> GPHMLNPQLVQPAKKPYNKIVSHLLVAEPEKIYAMPDPTVPDSDIKALTTLCDLADRELVVIIGWAKHIPGFSTLSLADQMS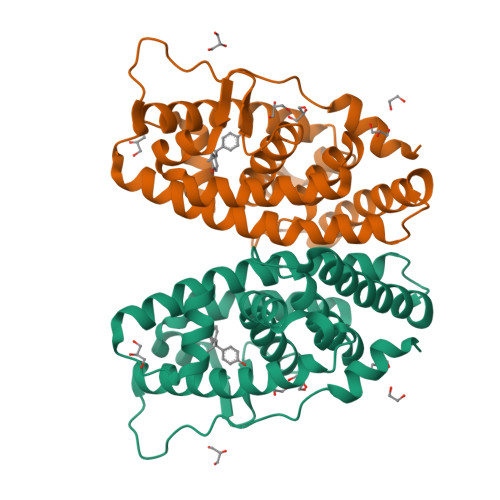LLQSAWMEILILGVVYRSLSFEDELVYADDYIMDEDQSKLAGLLDLNNAILQLVKKYKSMKLEKEEFVTLKAIALANSDSMHIEDVEAVQKLQDVLHEALQDYEAGQHMEDPRRAGKMLMTLPLLRQTSTKAVQHFYNIKLEGKVPMHKLFLEMLEAKV>[6x]GIDPFTMSLQEPVSPVEESPTSTADRIADLAARHEEAVVLAEKKAADRQHLKGKLTARARIDLLLDPGSFVELDEFVRHRTVEAGIPRPYGDGVVTGHGTIDGRQVCVFSHDFTTLGGSMGEAFGSKVVKI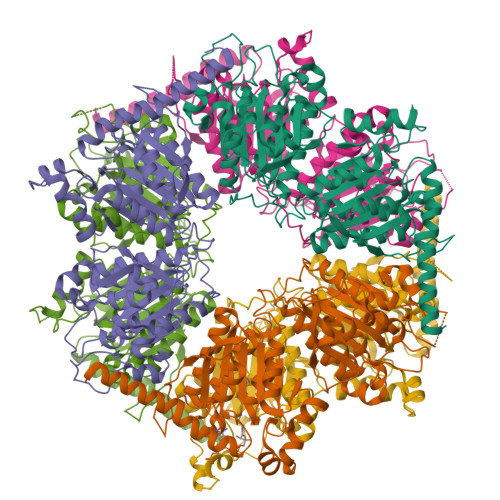YDFAMSVGCPVIGINDSGGARIQEGVMSIAYYTELGVRNVHSSGVIPQISLIMGPCAGGSVYSPALTDFTVMVKDISYMFVTGPEVVSAVMGEQVTAEQLGGPAVHAEVSGNAHYVGDDEQDAISWVQTLLGYLPPNNLDPAPVYDHDCAPGITEADLALDTVIPDSEQQVYDMADVITAVLDDGDYLEIHPDFARNIICALGRVEGHSVAVVANQPRHLAGVLDIDASEKAARFIRFCDSFNIPVLTFMDVPGYLPGVGQEHQGIIRRGIKLFYAYAESTVPKITVITRKAYGGGYAVMGSRQIGADRVMAWPTAEIAVMGANSAVPILHRRELAAVPPEERAAVKENLVDDYRRRFGNPYEAAAHGYVDMVISPSRTRYEVARALASLRNKRQARPARKHGNIPL> MGRNRIKKVTERLPLPPNARRVEDPEMNMSREVVEDPGVPGTQDVTFAVAEVNGVETGRLPVANVVVTPAHEAVVRVGTKPGTEVPPVIDGSIWDAIAGCEAGGNWAINTGNGYYGGVQFDQGTWEANGGLRYAPRADLATREEQIAVAE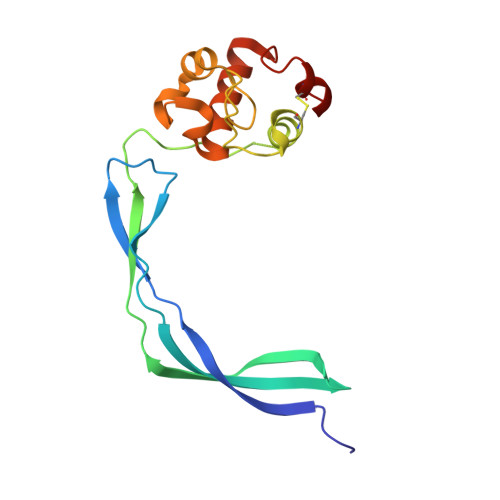VTRLRQGWGAWPVCAARAGAR>[2x]LTPAAESLNARWRTAVVDGWNNAFSGRYPFKNVSSDASLPLLAKYLNTDTGRIARFLQNNLSGVLHREGSRWVPDTINTRGLTFNPAFLK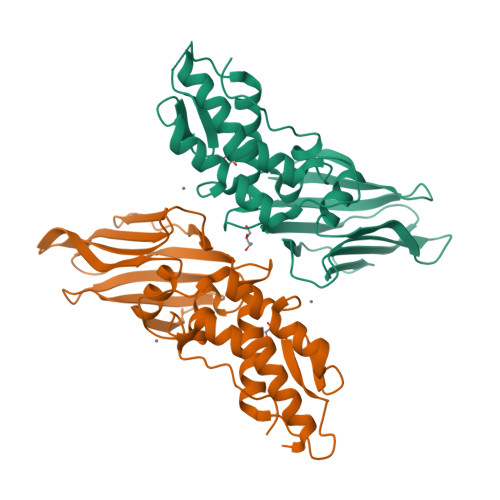AINTLSEIADVAFTTGNAGLHFELRPGTAAGVMQTTLITDNQKLIYVNQMPVWKRFTWPADTEAPGASLSWVSTQAGTRQYADLPGSWGLIRLLEMARRKAAPGVASGWSLSWQAQDGRMLNYTLRTEAGEGPLVLLKLRNFVLPETVFE>MRRFAAGCLALALLVLPFVLTGARAAEDESEKEIERYRQMIEDPMANPGFLNVDRGEVLWSEPRGTRNVSLETCDLGEGPGKLEGAYAHLPRYFADTGKVMDLEQRLLWCMETIQGRDTKPLVAKPFSGPGRTSDMEDLVAFIANKSDGVKIKVALATPQEKEMYAIGEALFFRRSSINDFSCSTCHGAAGKRIRLQALPQLDVPGKDAQLTMATWPTYRVSQSALRTMQHRMWDCYRQMRMPAPDYASEAVTALTLYLTKQAEGGELKVPSIKR[3x];>[3x]MRFETLLKRAAQVGALVLLPLAAHAQEASAVDPARVDAVVKTSFTKLPEGWESRLQQDETQRICSVTRNNPSPEQAAAIMKAEEVRIKFPAGPVLGSWKDGAKVAQNGRGGQFSDPPGTVSGGNCYACHQLD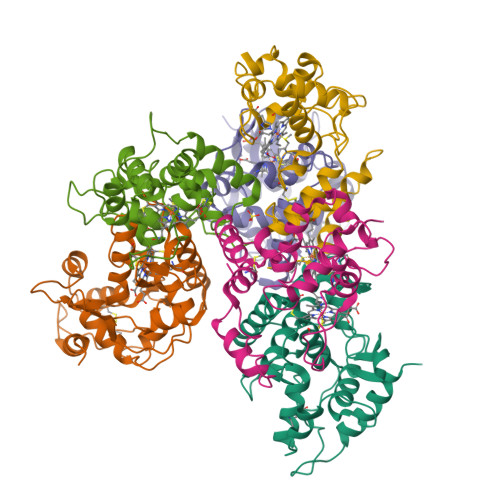PKEVSYGTLGPSLVGYGRERNFSAEDAKIAFAKVYDAQASLACSSMPRFGVNGVLTEQQIKDVVAYLFDPESPVNK> AAAAAAAAAAAAAAAAAAAAAAAAAAAAAAAAAAAAAIVINRMNNIQINPTSIGNPQTIRLPLNNFKSTTQLIQQVSLTDFFRPDIEHAGSTVLILRHPTDLPHLARHRAPPGRQTERLAEAWGQLLEASESGCARAYVTSLS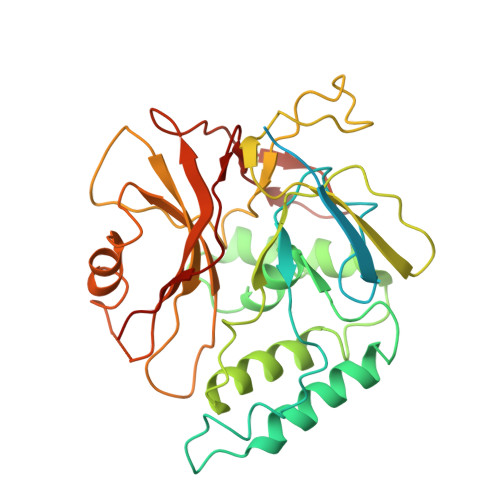FIAACRAEEYTDKQAAEANRTAIVSAYGCSRMGARLIRFSECLRAMVQCHVFPHRFISFFGSLLEYTIQDNLCNITAVAKGPQEAARTDKTSTRRVTANIPACVFWDVDKDLHLSADGLKHVFLVFVYTQRRQREGVRLHLALSQLNEQCFGRGIGFLLGARICMYAAYTLIGTIPSESVRYTRRMERFGGYNVPTIWLEGVVWGGTNTWNECY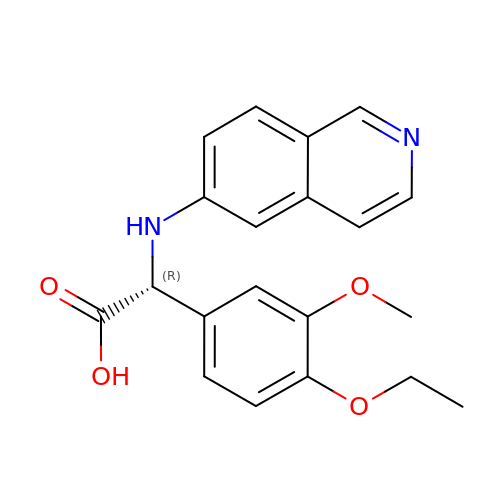(2~{R})-2-(4-ethoxy-3-methoxy-phenyl)-2-(isoquinolin-6-ylamino)ethanoic acid | C20 H20 N2 O4 | IHYCOARTGIZNKD-LJQANCHMSA-N>[4x]SMGKETPAKFFQYGLTPDRDGIIITRYLGKGIAVVLPSQIDGLPVVEVATK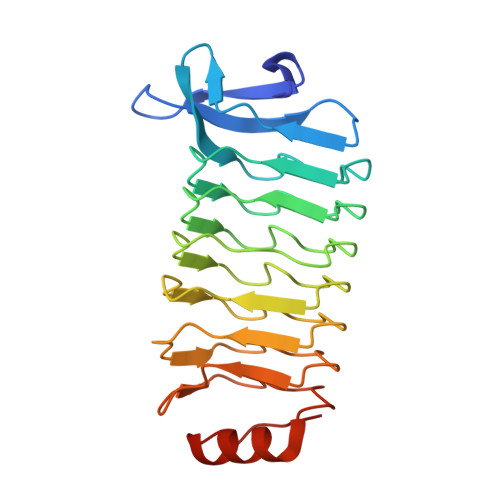AFYGCVSLVRVSLPSSVRMIGQHAFDGCTKLARIELPDGLREIRHHAFHKCVSLAGIVFPRSLQVIGQDVFSSCGSLVDVVLPNSVKEIGSGAFRDCAELASVRLPVGVKNLADGLFEGCRNLVELGNLPEKVSFGVGVFVGCYRLPDVLKRSVRKLGYKGEFAAA> MEKTDEYLLARFKGDGVKYKAKLIGIDDVPDARGDKMSQDSMMKLKGMAAAGRSQGQHKQRIWVNISLSGIKIIDEKTGVIEHEHPVNKISFIARDVTDNRAFGYVCGGEGQHQFFAIKTGQQAEP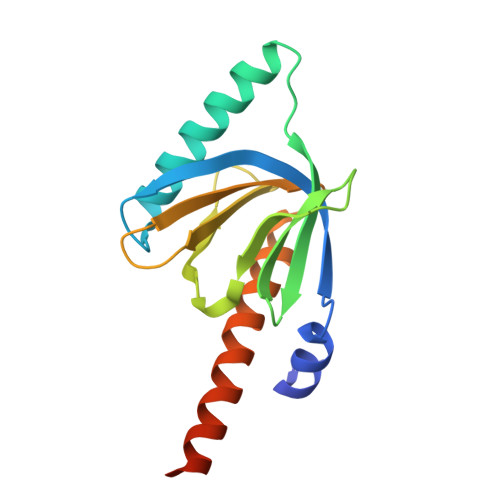LVVDLKDLFQVIYNVKKKEEDKKKVEEANKAEEN>ATTLKMGMQASVGSVEYNSAKMLADTLEEMSQGEIKLALYPSAQLGDDRAMLQQLTLGDLDITYAEFGRMGLWIPRAEAVMLPYVAKDFDHLRRMFESDFGQGVRDEMLQKFNWRALDTWYNGTRETTSNRPLNSIEDFKGLKLRVPNAKQNLNYAKLSGASPTPMSFSEVYLALQTNAVDGQENPLPTIKTMKFYEVQKNLAMTHHIVNDQMVIISESTWQKLSDTDKDIIQKAVQKVGDAHTQTVKTQEAELVSFFKSEGINVTYPDLEPFREAMQPLY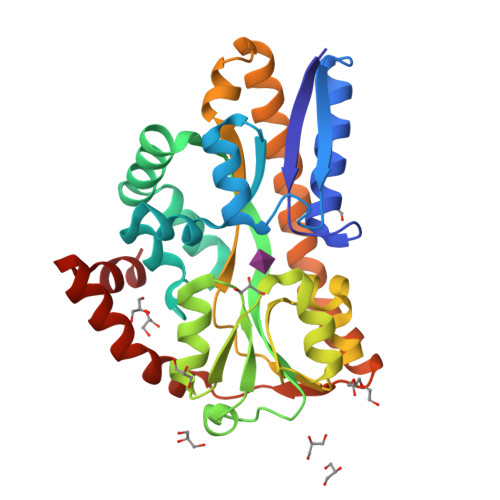KEFDSNIGQPIVSKLAAM[2x]NAMPT functions as a homo-dimeric enzyme that catalyzes the rate limiting step in the primary salvage pathway for NAD synthesis, the transfer of a phosphoribosyl residue from 5-phosphoribosyl-1-pyrophosphate (PRPP) to nicotinamide (NAM) to produce nicotinamide mononucleotide (NMN). Crystal structures of NAMPT in numerous ligand-bound forms have been reported. These structures consistently display a NAMPT homo-dimer with two essentially identical active sites at the dimer interface. Typical NAMPT inhibitors were found to occupy the portion of active site responsible for NAM binding and a tunnel-shaped cavity extending from the NAM binding site. Furthermore, we determine the crystal structures of six NAMPT mutants in the apo form and in complex with various inhibitors and present a definitive model to explain the differential effects of the mutations on various structural classes of NAMPT inhibitors.

However, the part of NAMPT structure that is responsible for inhibitor binding is not affected by the S165 mutations. This prompted us to investigate whether the mutations had effects on the phosphoribosylated (pRib) adduct of the inhibitors, because it has been shown that the cellular potency of NAMPT inhibitors is dependent on the formation of a pRib adduct and the resulting inhibitory activity of the compound adduct. We determined the crystal structures of NAMPT-S165F in complex with GNE-617, a close analogue of GNE 618, and its adduct pRib-GNE-617. These structures revealed that the pRib-GNE-617 binding converted 380GRS back into a helical conformation. The rewound helix, however, adopted a different orientation compared to the wild-type structure and avoided the steric clashed between Leu386 and Phe165. The dramatic conformational changes induced by binding the pRib-adduct suggested a significant energetic barrier and decreased inhibitory activity.

> MNPAAEAEFNILLATDSYKVTHYKQYPPNTSKVYSYFECREKKTENSKLRKVKYEETVFYGLQYILNKYLKGKVVTKEKIQEAKDVYKEHFQDDVFNEKGWNYILEKYDGHLPIEIKAVPEGFVIPRGNVLFTVENTDPECYWLTNWIETILVQSWYPITVATNFREQKKILAKYLLETSGNLDGLEYKLHDFGYRGVSSQETAGIGASAHLVNFKGTDTVAGLALIKKYYGTKDPVPGYSVPAAEHSTITAWGKDHEKDAFEHIVTQFSSVPVSVVSDSYDIYNACEKIWGEDLRHLIVSRSTQAPLIIRPDSGNPLDTVLKVLEILGKKFPVTENSKGYKLLPPYLRVIQGDGVDINTLQEIVEGMKQKMWSIENIAFGSGGGLLQKLTRDLLNCSFKCSYVVTNGLGINVFKDPVADPNKRSKKGRLSLHRTPAGNFVTLEEGKGDLEEYGQDLLHTVFKNGKVTKSYSFDEIRKNAQLNIELEAAHHLEHHHHHHHH>MSQQENPKYLWWNHRIIPWEEATVHLTDYWWASVTAVFEGIRGYWNNAEGEMYIFRLEDHARRLEQSMQLIRMPKEFTVDEICQATIDLVRANDYRGDVYIMPLAYAVGNKAFSVVGDRTTEMFIYSRPAVSRLEEDFSLHACYSSWTRINERVLPPRIKALANYRNSQLASSEAAMNGYDTALFLNPEGKVAEGTGSCVFFVRKGKLITPDITSGILESITRDTVIHLAREVLGLEVEERVVDRTETYLADEAFLCGTHAEITPIASIDR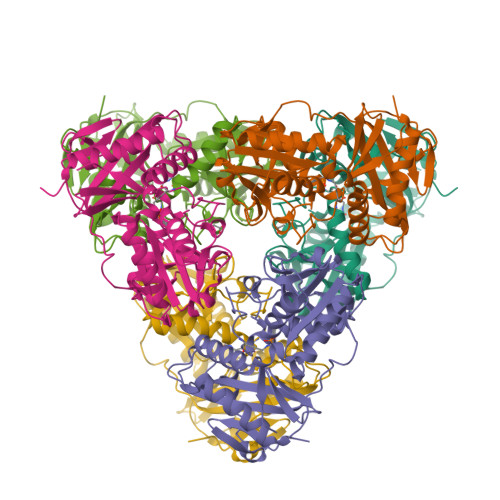HEMKHGAPGPITRQLRDIYREVVYGRDFRYRNWLTPVGMGVRAEQ[3x]>[3x]MKKLLPILIGLSLSGFSSLSQAENLMQVYQQARLSNPELRKSAADRDAAFEKINEARSPLLPQLGLGADYTYSNGYRDANGINSNATSASLQLTQSIFDMSKWRALTLQEKAAGIQDVTYQTDQQTLILNTATAYFNVLNAIDVLSYTQAQKEAIYRQLDQTTQRFNVGLVAITDVQNARAQYDTVLANEVTARNNLDNAVEQLRQITGNYYPELAALNVENFKTDKPQPVNALLKEAEKRNLSLLQARLSQDLAREQIRQAQDGHLPTLDLTASTGISDTSYSGSKTRGAAGTQYDDSNMGQNKVGLSFSLPIYQGGMVNSQVKQAQYNFVGASEQLESAHRSVVQTVRSSFNNINASISSINAYKQAVVSAQSSLDAMEAGYSVGTRTIVDVLDATTTLYNAKQELANARYNYLINQLNIKSALGTLNEQDLLALNNALSKPVSTNPENVAPQTPEQNAIADGYAPDSPAPVVQQTSARTTTSNGHNPFRN

Colicin E1 is a bacteriocin produced by, and lethal to, Escherichia coli that hijacks the outer membrane proteins (OMPs) TolC and BtuB to enter the cell. Colicin E1 is a bacteriocin produced by E. coli that enters the periplasm of neighboring cells and forms a pore on the cytoplasmic membrane leading to membrane depolarization and cell death. Unlike any of the other E colicins, the T domain of Colicin E1 binds to TolC, the outer membrane component of the acridine efflux pump, and the R domain binds BtuB, the primary receptor shared by all E colicins. TolC forms a large rigid conduit in the outer membrane and periplasm with a water-filled lumen.

We recently reported a high-yield TolC preparation by refolding from inclusion bodies and inserted refolded TolC into nanodiscs. The cryoEM structure of refolded TolC alone is similar to the previously published crystal structures of natively derived TolC alone or in complex with hexamminecobalt but with more splayed loops at the periplasmic opening (residues 165–175). There was local variation in resolution within the model with lower resolution associated with the extracellular/periplasmic ends and the nanodisc scaffold protein. The lower residue resolution at these apertures may indicate dynamics not captured in the X-ray crystal structures. When resolved by cryoEM, addition of ColE1-T to TolC breaks the threefold channel symmetry and the additional protein is observed running all the way through the TolC barrel as a single-pass, all-α-helical chain spanning more than 130 Å. The maps refined to nominal global resolutions of 2.84 Å and 3.09 Å for the TolC and ColE1-T:TolC, respectively (Figure 1—source data 1).>MSLANLSELPNIGKVLEQDLIKAGIKTPVELK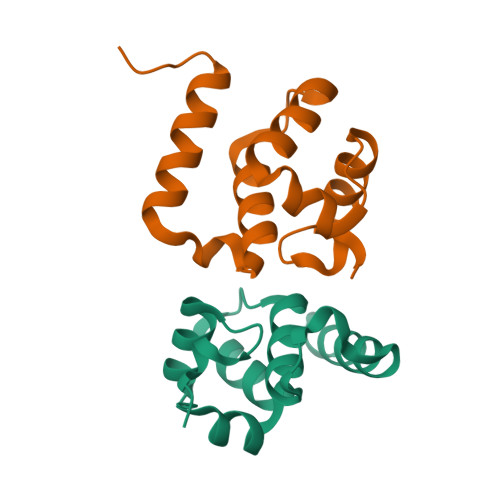DVGSKEAFLRIWENDSSVCMSELYALEGAVQGIRWHGLDEAKKIELKKFHQSLEGHHHHHH[2x]>[2x]MNVYRGVHELIGHTPIVEITRFSLPEGVRLFAKLEFYNPGGSVKDRLGRELIEDALEKGLVTEGGTIIEPTAGNTGIGLALAALQHDLRVIVCVPEKFSIEKQELMKALGATVVHTPTEQGMTGAIAKAKELVNEIPNSYSPSQFANEANPRAYFKTLGPELWSALNGEINIFVAGAGTGGTFMGTASYLKEKNIDIKTVIVEPEGSILNGGKAGSHETEGIGLEFI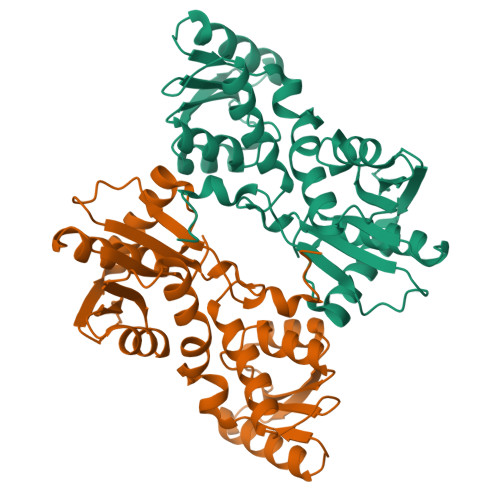PPFLKTSYFDEIHTISDRNAFLRVKELAQKEGLLVGSSSGAAFHASLLEAEKAAPGTNIVTIFPDSSERYLSKDIYKGWELEHHHHHH> GAMASELTPEERSELKNSIAEFHTYQLDPGSCSSLHAQRIHAPPELVWSIVRRFDKPQTYKHFIKSCSVEQNFEMRVGCTRDVIVISGLPANTSTERLDILDDERRVTGFSIIGGEHRLTNYKSVTTVHRFEKENRIWTVVLESYVVDMPEGNSEDDTRMFADTVVKLNLQKLATVAEAMARNSGDGSGSQVT;> GAMGRSVYELDCIPLWGTVSIQGNRSEMEDAFAVSPHFLKLPIKMLMGDHEGMSPSLTHLTGHFFGVYDGHGGHKVADYCRDRLHFALAEEIE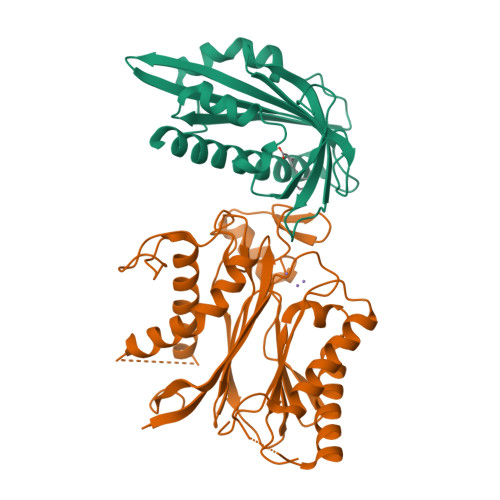RIKDELCKRNTGEGRQVQWDKVFTSCFLTVDGEIEGKIGRAVVGSSDKVLEAVASETVGSTAVVALVCSSHIVVSNCGDSRAVLFRGKEAMPLSVDHKPDREDEYARIENAGGKVIQWQGARVFGVLAMSRSIGDRYLKPYVIPEPEVTFMPRSREDECLILASDGLWDVMNNQEVCEIARRRILMWHKKNGAPPLAERGKGIDPACQAAADYLSMLALQKGSKDNISIIVIDLKAQRKFKTRT>[2x]GSSMVTGGMASKWDQKGMDIAYEEAALGYKEGGVPIGGCLINNKDGSVLGRGHNMRFQKGSATLHGEISTLENCGRLEGKVYKDTTLYTTLSPCDMCTGAIIMYGIPRCVVGENVNFKSK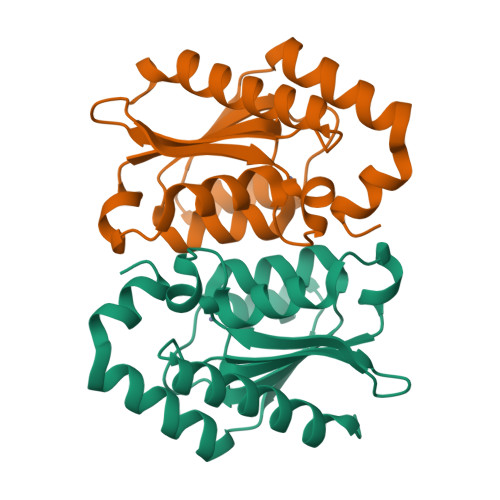GEKYLQTRGHEVVVVDDERCKKIMKQFIDERPQDWFEDIGE>NYLFEYAPDVLESFPNKHVNRDYFVKFNCPEFTSLCPKTGQPDFATIYISYIPDEKMVESKSLKLYLFSFRNHGDFHQDCMNIIMNDLIELMDPRYIEVWGKFTPRGGISIDPYTNYGKPGTKYEKM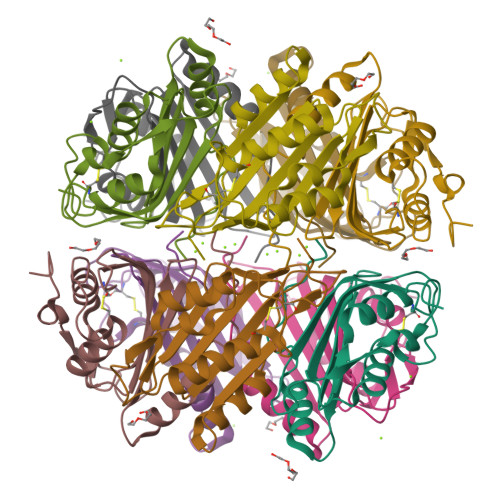AEYRMMNHDLYPETIDNR[5x]>[2x]MASKPQPIAAANWKCNGSESLLVPLIETLNAATFDHDVQCVVAPTFLHIPMTKARLTNPKFQIAAQNAITRSGAFTGEVSLQILKDYGISWVVLGHSERRL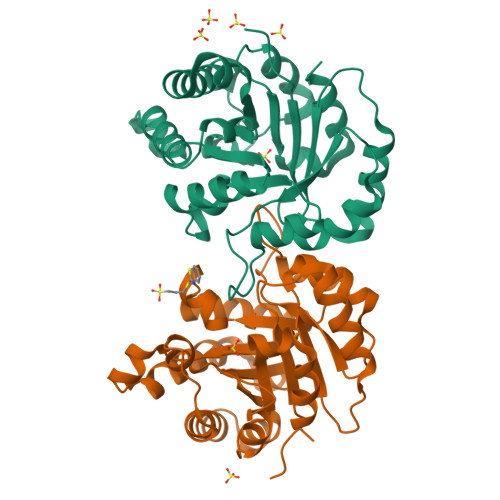YYGETNEIVAEKVAQACAAGFHVIVCVGETNEEREAGRTAAVVLTQLAAVAQKLSKEAWSRVVIAYEPVWAIGTGKVATPQQAQEVHELLRRWVRSKLGTDIAAQLRILYGGSVTAKNARTLYQMRDINGFLVGGASLKPEFVEIIEATK> GAMANHLRAEGPASVLAIGTANPENILLQDEFPDYYFRVTKSEHMTQLKEKFRKICDKSMIRKRNCFLNEEHLKQNPRLVEHEMQTLDARQDMLVVEVPKLGAMANHLRAEGPASVLAIGTANPENILLQDEFPDYYFRVTKSEHMTQLKEKFRKICDKSMIRKRNCFLNEEHLKQNPRLVEHEMQTLDARQDMLVVEVPKLGKDACAKAIKEWGQPKSKITHLIFTSASTTDMPGADYHCAKLLGLSPSVKRVMMYQLGCYGGGTVLRIAKDIAENNKGARVLAVCCDIMACLFRGPSESDLELLVGQAIFGDGAAAVIVGAEPDESVGERPIFELVSTGQTILPNSEGTIGGHIREAGLIFDLHKDVPMLISNNIEKCLIEAFTPIGISDWNSIFWITHPGGKAILDKVEEKLHLKSDKFVDSRHVLSEHGNMSS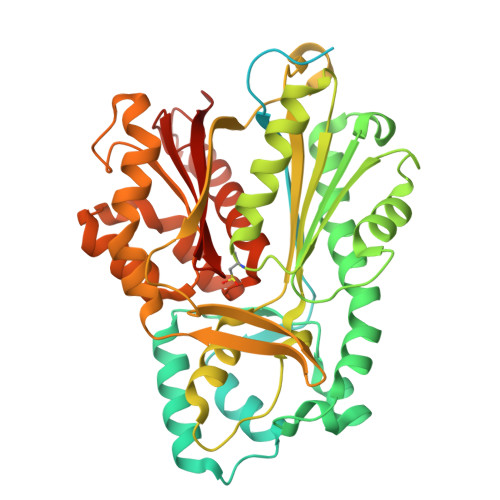STVLFVMDELRKRSLEEGKSTTGDGFEWGVLFGFGPGLTVERVVVRSVPIKY> MGSDKIHHHHHHMKEIDELT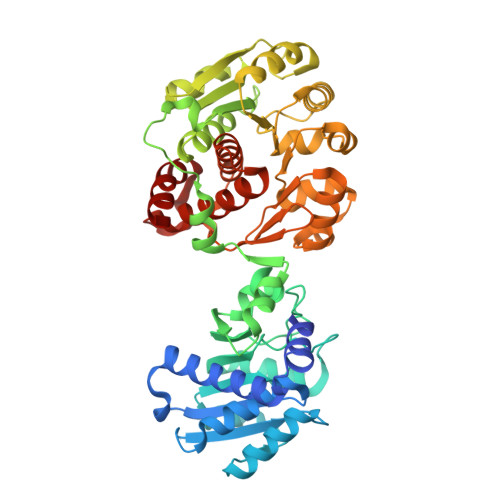IKEYGVDSRILMERAGISVVLAMEEELGNLSDYRFLVLCGGGNNGGDGFVVARNLLGVVKDVLVVFLGKKKTPDCEYNYGLYKKFGGKVVEQFEPSILNEFDVVVDAIFGTGLRGEITGEYAEIINLVNKSGKVVVSVDVPSGIDSNTGKVLRTAVKADLTVTFGVPKIGHILFPGRDLTGKLKVANIGHPVHLINSINRYVITREMVRSLLPERPRDSHKGTYGKVLIIAGSRLYSGAPVLSGMGSLKVGTGLVKLAVPFPQNLIATSRFPELISVPIDTEKGFFSLQNLQECLELSKDVDVVAIGPGLGNNEHVREFVNEFLKTLEKPAVIDADAINVLDTSVLKERKSPAVLTPHPGEMARLVKKTVGDVKYNYELAEEFAKENDCVLVLKSATTIVTDGEKTLFNITGNTGLSKGGSGDVLTGMIAGFIAQGLSPLEASTVSVYLHGFAAELFEQDERGLTASELLRLIPEAIRRLKE>[13x]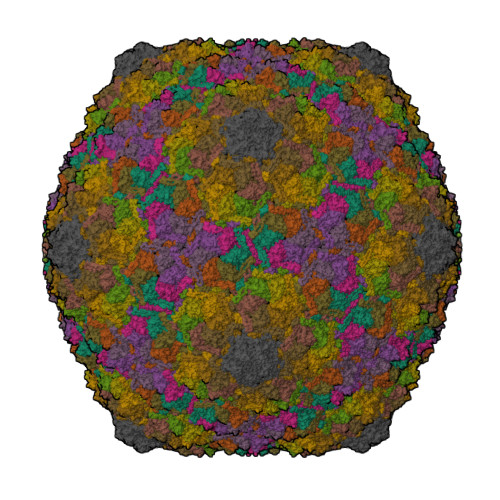AVNQSSSVEVSSESYETIFSQRIIRDLQKELVVGALFEELPMSSKILTMLVEPDAGKATWVAASTYGTDTTTGEEVKGALKEIHFSTYKLAAKSFITDETEEDAIFSLLPLLRKRLIEAHAVSIEEAFMTGDGSGKPKGLLTLASEDSAKVVTEAKADGSVLVTAKTISKLRRKLGRHGLKLSKLVLIVSMDAYYDLLEDEEWQDVAQVGNDSVKLQGQVGRIYGLPVVVSEYFPAKANSAEFAVIVYKDNFVMPRQRAVTVERERQAGKQRDAYYVTQRVNLQRYFANGVVSGTYAAS 neo-Inositol pentakisphosphate 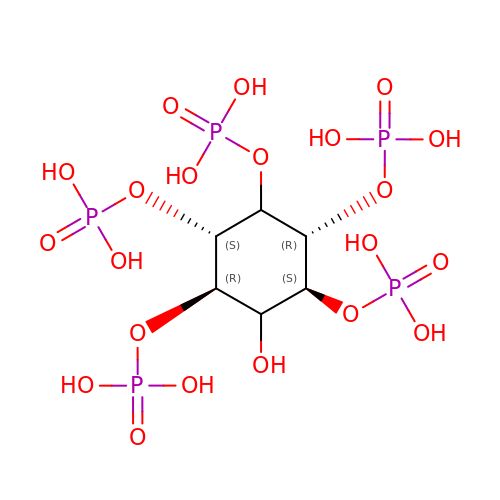| C6 H17 O21 P5 | CTPQAXVNYGZUAJ-WJVUKCJRSA-N>GKELRQLQEDRKNDKKPPPYKHIKVNRPIGRVQIFTADLSEIPRCNCKATDENPCGIDSECINRMLLYECHPTVCPAGGRCQNQCFSKRQYPEVEIFRTLQRGWGLRTKTDIKKGEFVNECVGELIDEEECRARIRYAQEHDITNFYMLTLDKDRIIDAGPKGNYARFMNHCCQPNCETQKWSVNGDTRVGLFA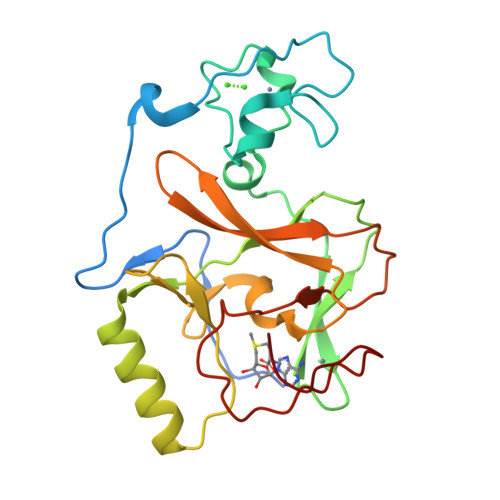LSDIKAGTELTFNYNLECLGNGKTVCKCGAPNCSGFLG[2x]>MHHHHHHKNIINTSILNLRYESNHLIDLSRYASEINIGSKVNFDPIDKNQIQLFNLESSKIEIILKNAIVYNSMYENFSTSFWIKIPKYFSKINLNNEYTIINCIENNSGWKVSLNYGEIIWTLQDNKQNIQRVVFKYSQMVAISDYINRWIFITITNNRLNNSKIYINGRLIDQKPISNLGNIHASNNIMFKLDGCRDPHRYIWIKYFNLFDKELNEKEIKDLYDNQSNSGILKDFWGNYLQYDKPYYMLNLYDPNKYVDVNNVGIR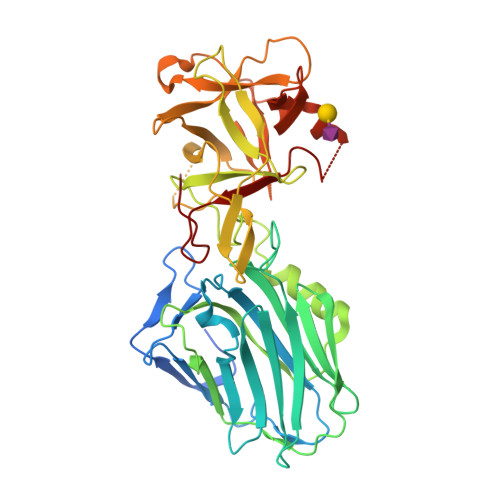GYMYLKGPRGSIVTTNIYLNSSLYMGTKFIIKKYASGNKDNIVRNNDRVYINVVVKNKEYRLATNASQAGVEKILSVLEIPDVGNLSQVVVMKSKNDQGIRNKCKMNLQDNNGNDIGFIGFHQFNNIDKLVASNWYNRQIERSSRTFGCSWEFIPVDDGWGESPL[2x]[(2R,5S)-5-(4-amino-2-oxopyrimidin-1(2H)-yl)-1,3-oxathiolan-2-yl]methyl trihydrogen diphosphate | C8 H13 N3 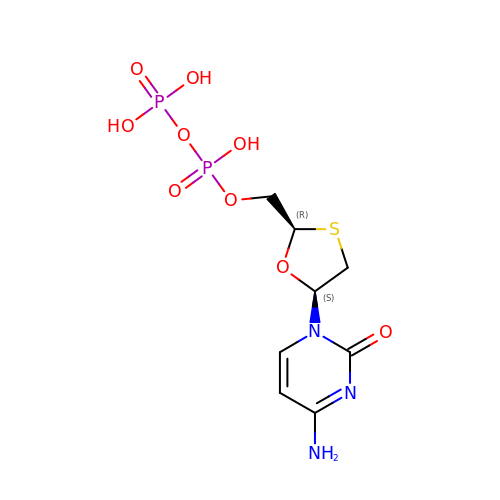O9 P2 S | AAHOBGDTTMOZKD-NKWVEPMBSA-N> MDSYSAPESTPSASSRPEDYFIGATPLQKRLESVRKQSSFILTPPRRKIPQCSQLQEDVDPQKVAFLLHKQWTLYSLTPLYKFSYSNLKEYSRLLNAFIVAEKQKGLAVEVGEDFDIKVIFSTLLGMKGTQRDPEAFLVQIVSKSQLPSENREGKVLWTGWFCCVFGDSLLETVSEDFTCLPLFLANGAESNTAIIGTWFQKTFDCYFSPLAINAFNLSWMAAMWTACKMDHYVATTEFLWSVPCSPQSLDISFAIHPEDAKALWDSVHKTPGEVTQEEVDLFMDCLYSHFHRHFKIHLSATRLVRVSTSVASAHTDGKIKILCHKYLIGVLAYLTEL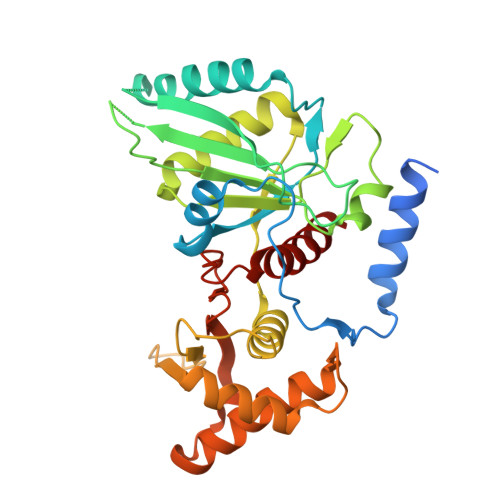AIFQIE pmcATP-binding cassette (ABC) transporters are ubiquitous membrane proteins that couple the energy of ATP binding and hydrolysis to the translocation of a wide variety of molecules across biological membranes. Here, we investigated whether a large separation of the nucleotide-binding domains is required for the transport cycle of BmrA, a homodimeric multidrug ABC transporter from Bacillus subtilis. Upon ATP binding, the NBDs engage in a transient tight dimer where the two nucleotides are sandwiched between the Walker A motif from one NBD and the ABC signature motif from the other NBD, thereby generating the OF conformation that is prone to drug release. Overall, our data suggest that the NBDs of BmrA function with a tweezers-like mechanism distinct from the related lipid A exporter MsbA.

We then introduced the A582C mutation into a cysteine-less mutant of BmrA replacing the single native cysteine at position 436 by a serine. For this purpose, we introduced by site-directed mutagenesis a cysteine residue near the C-terminal end of the NBD to restrain the separation between the two NBDs during the catalytic cycle and analyzed the impact of the disulfide-bond formation on the ATPase and transport activities of BmrA. We determined by cryo-EM the structure of the oxidized A582C mutant at 3.14 Å resolution. Consistent with its ability to transport drugs, the mutant displays a canonical IF conformation similar to that seen in related multidrug ABC transporters from the type IV subfamily. Interestingly a clear density bridging the two monomers is visible at the lower part of the two NBDs. This allows us to build the disulfide bond between the two Cys582 residues. As both were solved at identical resolution, it is presumably the cross-link bridge between the two monomers that rigidifies the C-terminal region of the mutant transporter. This allows us to build an additional ten residues in the oxidized C436S/A582C mutant structure. The transmembrane helices are perfectly superposed (rmsd of 0.45 Å over 549 residues) while the NBDs are slightly less separated in the mutant structure. We found that the presence of the disulfide bond between the NBDs did not prevent the ATPase activity nor the transport of drugs, demonstrating that a large separation of the NBDs is not mandatory for the transport function.

>[2x]MPTKKQKSKSKLKPFFALVRRTNPSYGKLAFALALSVVTTLVSLLIPLLTKQLVDGFSMSNLSGTQIGLIALVFFVQAGLSAYATYALNYNGQKIISGLRELLWKKLIKLPVSYFDTNASGETVSRVTNDTMVVKELITTHISGFITGIISVIGSLTILFIMNWKLTLLVLVVVPLAALILVPIGRKMFSISRETQDETARFTGLLNQILPEIRLVKASNAEDVEYGRGKMGISSLFKLGVREAKVQSLVGPLISLVLMAALVAVIGYGGMQVSSGELTAGALVAFILYLFQIIMPMGQITTFFTQLQKSIGATERMIEILAEEEEDTVTGKQIENAHLPIQLDRVSFGYKPDQLILKEVSAVIEAGKVTAIVGPSGGGKTTLFKLLERFYSPTAGTIRLGDEPVDTYSLESWREHIGYVSQESPLMSGTIRENISYGLERDVTDAEIEKAAEMAYALNFIKELPNQFDTEVGERGIMLSGGQRQRIAIARALLRNPSILMLDEATSSLDSQSEKSVQQALEVLMEGRTTIVIAHRLSTVVDADQLLFVEKGEITGRGTHHELMASHGLYRDFAEQQLKMNCDLENKAGVDKLAAALEHHHHHH> NKGTDDATADSRKTYTLTDYLKNTYRLKLYSLRWISDHEYLYKQENNILVFNAEYGNSSVFLENSTFDEFGHSINDYSISPDGQFILLEYNYVKQWRHSYTASYDIYDLNKRQLITEERIPNNTQWVTWSPVGHKLAYVWNNDIYVKIEPNLPSYRITWTGKEDIIYNGITDWVYEEEVFSAYSALW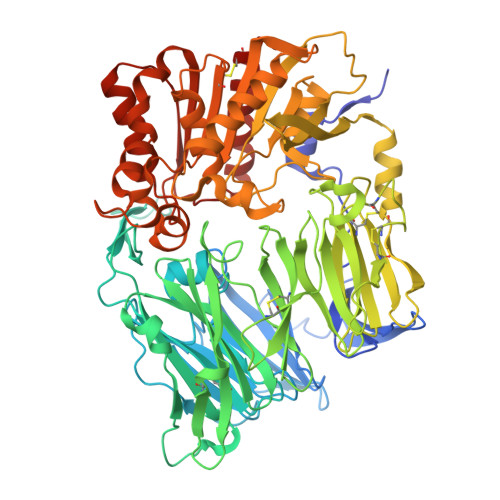WSPNGTFLAYAQFNDTEVPLIEYSFYSDESLQYPKTVRVPYPKAGAVNPTVKFFVVNTDSLSSVTNATSIQITAPASMLIGDHYLCDVTWATQERISLQWLRRIQNYSVMDICDYDESSGRWNCLVARQHIEMSTTGWVGRFRPSEPHFTLDGNSFYKIISNEEGYRHICYFQIDKKDCTFITKGTWEVIGIEALTSDYLYYISNEYKGMPGGRNLYKIQLSDYTKVTCLSCELNPERCQYYSVSFSKEAKYYQLRCSGPGLPLYTLHSSVNDKGLRVLEDNSALDKMLQNVQMPSKKLDFIILNETKFWYQMILPPHFDKSKKYPLLLDVYAGPCSQKADTVFRLNWATYLASTENIIVASFDGRGSGYQGDKIMHAINRRLGTFEVEDQIEAARQFSKMGFVDNKRIAIWGWSYGGYVTSMVLGSGSGVFKCGIAVAPVSRWEYYDSVYTERYMGLPTPEDNLDHYRNSTVMSRAENFKQVEYLLIHGTADDNVHFQQSAQISKALVDVGVDFQAMWYTDEDHGIASSTAHQHIYTHMSHFIKQCFSLP> MCTRVFDVSQRFILLVSLPPLSLSLRPSCCSRKAATRRRRSTASVLLATDALSLFVRTHYPSPLLFLLLPNFPLPIHSPRKQMRAAVGAVLQPSSSVGALRCQARFITRLYTSYFKGELFPNQLARPLERLPRGVSLAAARKGQQAAAPSSSGSGNPATTASLDVVTWGDVDSTDLVHANEQSRAVAPQAGLAPRRPYVPLGEVAKLELQGDYLTEGGLHQEALEYYGVVAKAYELAYPKDHPQVAGIRLKLAGAFRRTGRLTSSKANCEAVLQMLDSAVQPPLELIVEALFELGLTSEAMSDAAAGTVFEEAVALVDMFHNSGQSHKMLRLLPRLGRRFNLNFEEKFVYFSPFDYDRVFALADQCLERAEVFYQARNDRAGVMRVLQQR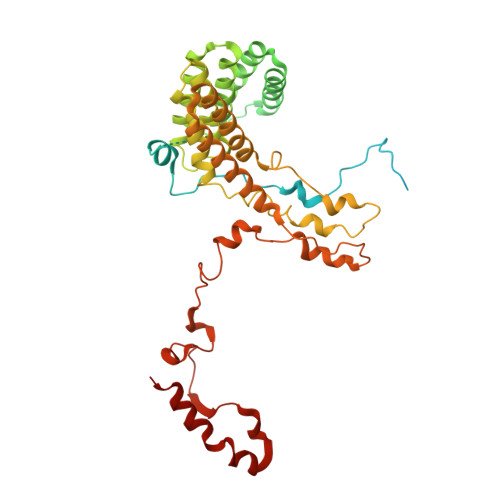KELIDKKFFNMRDFAGRIHTMRGHWKRRAQVLTNAPTPDELLRYSPTIHQVYRDFKYELNAPIGREKEVQPGVNRVVHDMGNPYRRSGVRSQRMFRDAEKNFEKYIRADAFEA Mitochondrial proteins CHCHD10 and CHCHD2 are mutated in rare cases of heritable FTD, ALS and PD and aggregate in tissues affected by these diseases. Here, we demonstrate that the low complexity N-terminal domains of both D10 and D2, as well as the full-length proteins, can form amyloid fibrils in vitro and in vivo. Structures of D10 and D2 fibrils assembled in vitro from the low complexity N-terminal domains of each protein show that their core comprises the most highly conserved region between the two proteins. For D10 and D2, the central conserved VAV motif forms a beta-strand that is associated with the protofilament interface in all the structures we have observed, suggesting that it may be a critical element in fibril formation and may be expected to appear in ex vivo structures as well.

We also determined the structure of D2-NT amyloid fibrils to 2.03 Å resolution, which again contains two identical PFs related by a helical symmetry axis. The core ordered region of each D2-NT PF consists of D2 residues G54–G86. A sequence alignment of D10 and D2 shows that this region corresponds to residues G43–G75 of D10 and features only 5 sequence differences between the two proteins. Therefore, the core ordered regions of D2-NT and D10-NT fibrils are formed by highly homologous regions within each protein. While the D2-NT PF fold differs from those of all three D10-NT PFs, certain elements are conserved. The D2 PF fold contains three strands consisting of residues L55–T61, V66–V68, and S70–T81. Strand-1 adopts a very similar conformation to that observed in the D10-NT PF1 structure, as do the last five residues of strand-3, and the two strands pack together in a nearly identical manner in both structures, with residue F73(D10)/F84(D2) packing against the equivalent Q47(D10)/Q58(D2) residue. However, in the D2-NT structure, strand-1 of one PF (PF-A) packs against strand-3 of the other PF (PF-B), because the beta-helix that connects the two strands in the D10-NT structure reverses on itself, allowing the C-terminal region of D2-NT PF-A to occupy the location of the C-terminal region of PF-B in the D10-NT structure. In addition to this, strand-2 of the D2-NT is superposable on the corresponding VAV sequence of all three D10-NT PFs and forms the central part of the PF interface both in the D2-NT structure and in D10-NT polymorph-1. Notably, the five sequence variations in the core ordered region of D2 compared with D10 occur either at positions facing the outside of the D2-NT fibril structure (D2 residues L76, H78 and I80), or are isosteric to (T75 in D2 vs. V64 in D10) or smaller than (G83 in D2 vs. A72 in D10) the corresponding residues in D10.

>MPRGSRSRTSRMAPPASRAPQMRAAPRPAPVAQPPAAAPPSAVGSSAAAPRQPGLMAQMATTAAGVAVGSAVGHTLGHAITGGFSGGSNAEPARPDITYQEPQGTQPAQQQQPM[6x]4-methoxy-1H-indole | C9 H9 N O | 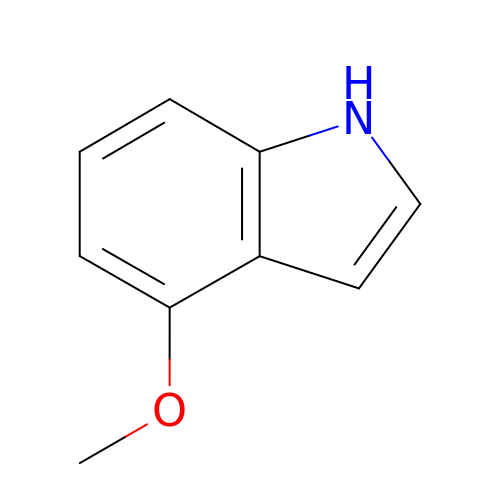LUNOXNMCFPFPMO-UHFFFAOYSA-N> MHPVERKSQSAPARLITRYRKQLPYINFYRFCQLLEQSQPDQPPI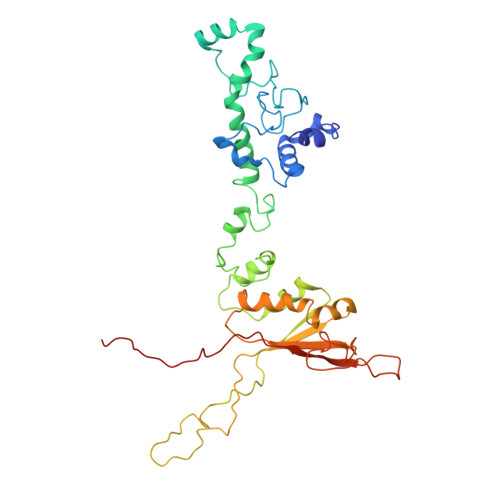GSGWQARQEAVRFCPYPGMGFPASEIKDAVIPEESHLPPIVHVTFMGLYGVTSPLPAHYISDIAQQREGHEAAADFLDIFSHRLITQYYRIWRKYSYPATFEAGGQDKTSQYLLGLARLGIPGCAQNIATPVSRFLALLPLMLLPGRTAEGLTSLVTLLAPGTQARVWHHDRRRIPLKTPLTMRVHHPVSLKSRPVMGDHATDVNGQVLLQLSTQTGSEVQGWLPGGHLYSDLLALLHVYLGSRLDVRLQLCVERSLLPDARLSCRPAAGSPQLGRTAVMRTQAKIATSAARVMTISLGRYQRVQEHYQRKETQENGDYRW> GHMGNQFVMPDLSGMFWVDAEPRLRALGWTGMLDKGADVDAGGSQHNRVVYQN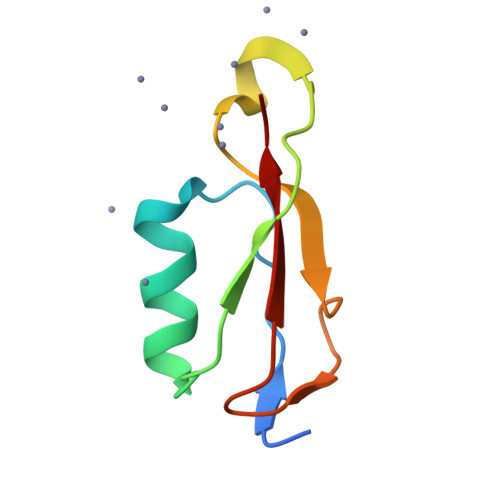PPAGTGVNRDGIITLRFGQ5-[4-(1H-indol-3-yl)butoxy]-1-phenyl-1H-pyrazole-4-carboxylic 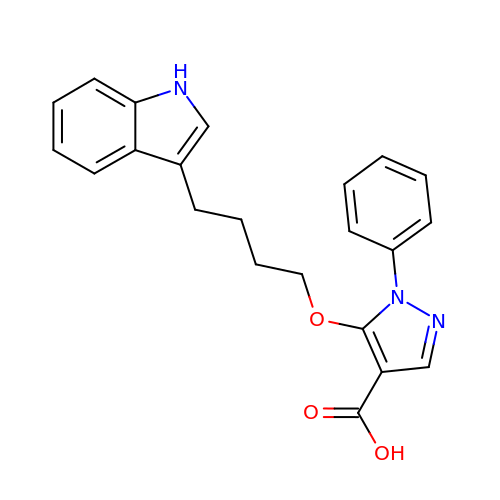acid | C22 H21 N3 O3 | AETXYNJTNADCGV-UHFFFAOYSA-N3-[4-(piperidin-1-ylmethyl)phenyl]-9H-pyrrolo[2,3-b:5,4-c']dipyridine-6-carbonitrile 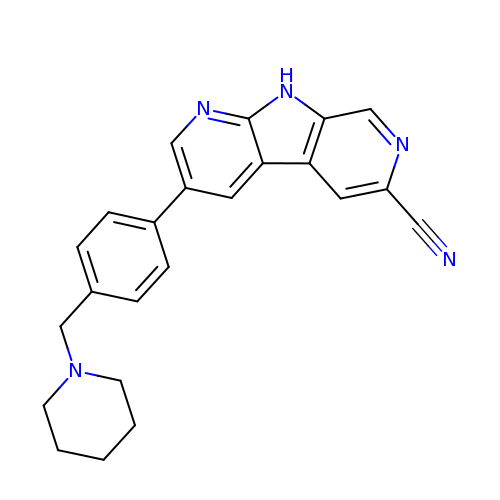| C23 H21 N5 | PPYHOOZGDDPLKM-UHFFFAOYSA-N> IDLSRERDPNFFDHPGIPVPECFWFMFKNNVRQDAGTC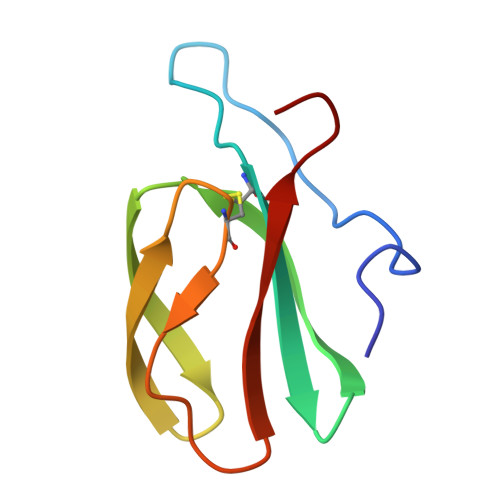YSSWKMDMKVGPNWVHIKSDDNCNLSGDFPPGWIVLGKKRPGF>[4x]MEDGKRLRIGITLHPYYSYVSNIVGDKAEVVPLIPAGFNPHAYEPRAEDIKRIGTLDVVVLNGVGHDDFAERMIASSEKPGIPVIEANAKVPLLAATGMAARGAGKVVNPHTFLSISASITQVNTIAR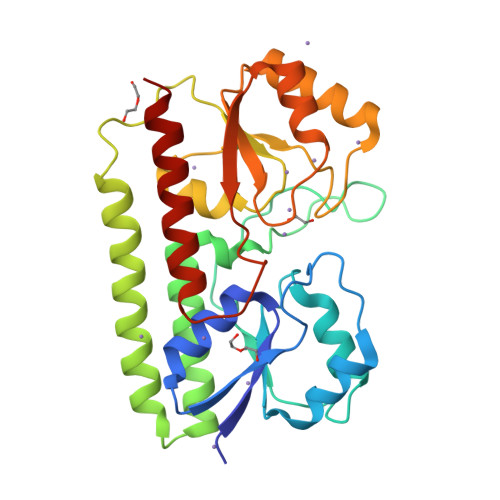ELGKLDPANAKAYTRNARAYAKRLRALRADALARLNKAPAADFRVATIHGAYDYLLREFGLEVTAVVEPAHGIEPSPSQLKKTIDQLKALDVKVIFSEIDFPSTYVETIQRESGVKLYSLSHISYGDYSAGKYEEEMARNLDTVVRAIQESGA>[2x]AHQDALPRLPVPPLQQSLDYYLKALQPIVSEEEWAHTKQLVDEFQTSGGVGERLQKGLERRAKKMENWLSEWWLKTAYLQFRQPVVIYSSPGVILPKQDFVDLQGQLRFAAKLIEGVLDFKSMIDNETLPVEFLGGQPLCMNQYYQILSSCRVPGPKQDSVVNFLKSKRPPTHITVVHNYQFFELDVYHSDGTPLTSDQIFVQLEKIWNSSLQSNKEPVGILTSNHRNTWAKAYNNLIKDKVNRESVNSIQKSIFTVC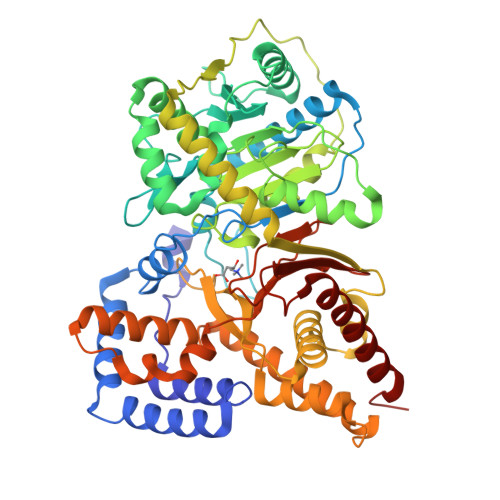LDKQVPRVSDDVYRNHVAGQMLHGGGSKFNSGNRWFDKTLQFIVAEDGSCGMVYEHAAAEGPPIVALVDHVMEYTKKPELVRSPMVPLPMPKKLRFNITPEIKNDIEKAKQNLSIMIQDLDIMMLTFHHFGKDFPKSEKLSPDAFIQVALQLAYYRIYGQACATYESASLRMFHLGRTDTIRSASIDSLAFVKGMGDSTVPEQQKVELLRKAVQAHRAYTDRAIRGEAFDRHLLGLKLQAIEDLVSMPDIFMDTSYAIAMHFNLSTSQVPAKTDCVMFFGPVVPDGYGICYNPMEAHINFSVSAYNSCAETNAARMAHYLEKALLDMRTLLQNHPRAK>[4x]ALESAQESHALHHQNAAALRFQFHITREQAREIVKLCPNCPDWGHAPQLGVNPRGLKPRVLWQMDVTHVSEFGKLKYVHVTVDTYSHFTFATARTGEATKDVLQHLAQSFAYMGIPQKIKTDNAPAYVSRSIQEFLARWKISHVTGIPYNPQGQAIVERTHQNIKAQLNKLQKAGKYYTPHHLLAHALFVLNHVNMDNQGHTAAERHWGPISADPKPMVMWKDLLTGSWKGPDVLITAGRGYA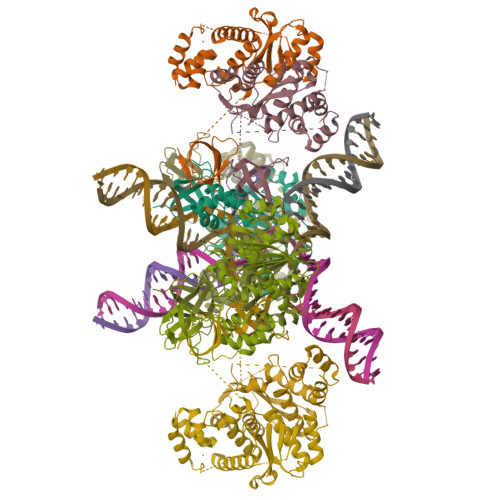CVFPQDAESPIWVPDRFIRPFTERKEATPTPGTAEKTPPRDEKDQQESPKNESSPHQREDGLATSAGVDLRSGGGP> HMDVEQLGRSSWTLLHSVAASYPAQPTDQQKGEMKQFLNIFSHIYPCNWCAKDFEKYIRENAPQVESREELGRWMCEAHNKVNKKLRKPKFDCNFWE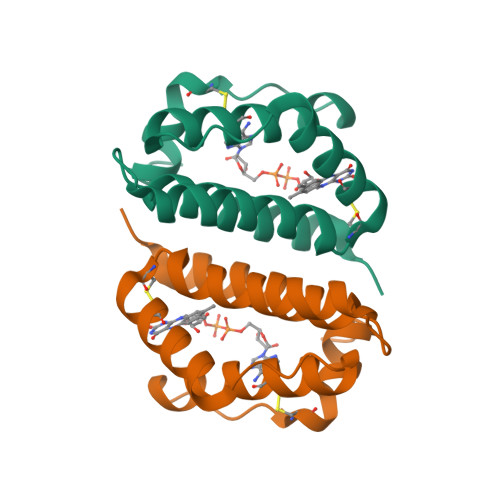KRWKDGWDE> MSLAKVWTYASWIPRGIPKAMANELSSAAAALAHPEAIARVAQLESQGKNPYRVARAEFWQMYLACWPYRFRNTVVEWETCKAKVLKGSVDLQDIVDLLYLLAWAYLFWILGEIYGRGSLYGYRFDGEIHRQEAQNVILYKEKEAQEMAVVMEKLEKEIQEWLKTMEQE;> MPGGGTIRFWREKLEGYKKYHQIVKTIKMVTLAKYRQTVVRTRVRDQTLRYTRKALDAKTQDDQEVIEKSECLLYVPITTNRGSCGALNTNMVRYLQEVENPKMTIISVGKKALDAMTKVFQDTYRRTILNDMKQAMSFQFAAYVLEHMNTVPWDRAQIVYNRYHGAASQKLAIFNLPKFEDWKQKLEEDSAGDGKIEEDGLLQSLPMKTALGELEETAVEDFYNFHSCLAVLNAVSENELSEYAARIVAVENQLGNITGLMQLADYTYNKTRKELITAELLEIIGTMTAMHAGKKVGLKKTEFWK;> MRASRTLLLSVSRFMRQDPRKFFPDNGFRFFDGPEDSFGDGNIPAQIILTLTRQDEFILKQEPVAAITIRTNEGEMGVLAGHEYTVQQLAPGILEVEYEGGKKDQYVISGGFAHVNDTGVVDINTVEAVPLEEIDHEKLAKALEEARAKSQSPDEAVRIQGEI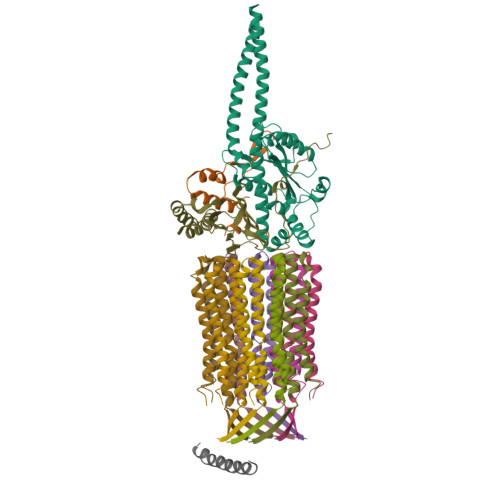ALEIFEPLEAALH;> MSWRDAGISYLRYLSIVTRCIHEVQKEGPLLTKNVRFSTIGWKSLYLDHGATKEYTAIPAELEKIPENQVAQQHHA;>MQRGSSITKVVRRAALARSTRNAAIAYEVTVNGANLIGAGMAASGVGVPAIGVAMCFSSYMLAAARQPNMSAKLLPYCILGFALSEALALFTLLIALLELFVFS[10x]>[6x]NPCLTGPRTCKDLLDRGHFLSGWHTIYLPDCRPLTVLCDMDTDGGGWTVFQRRVDGSVDFYRDWATYKQGFGSRLGEFWLGNDNIHALTAQGTSELRTDLVDFEDNYQFAK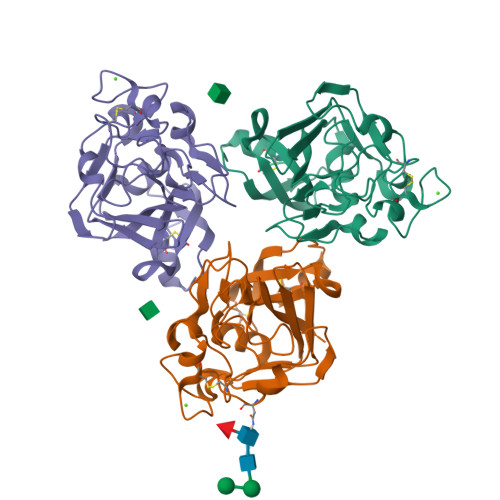YRSFKVADEAEKYNLVLGAFVEGSAGDSLTFHNNQSFSTKDQDNDLNTGNCAVMFQGAWWYKNCHTSNLNGRYLRGTHGSFANGINWKSGKGYNYSYKVSEMKVRPA> MKKLVMTAAVAAILGAASPVMAQGIPVFDGTRALDFVQQFARMKEQLDTAKDQLAEAQRMYEAVTGGRGLGDLMRNAQLREYLPDDLRTVYDSANGGGYSGISGSINDILRDERLNGSVADMRRSIEERSRTAAATDKAVGLRAYEGAQQRLAQIEGLMDEISRTQDQKAIEELQARIAGEQAAIQNETTKLQMIAQLRQAEQALIS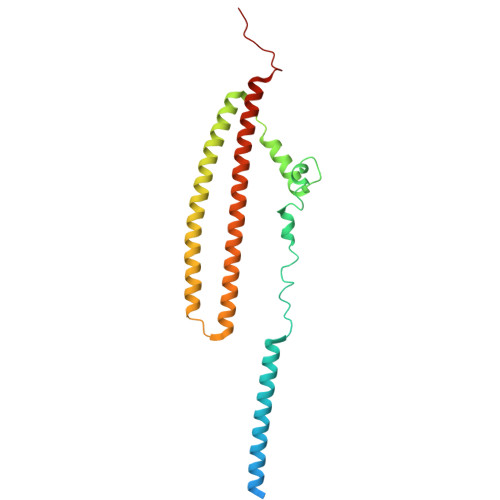EQRRERNMRILSSGNQGMPTIQ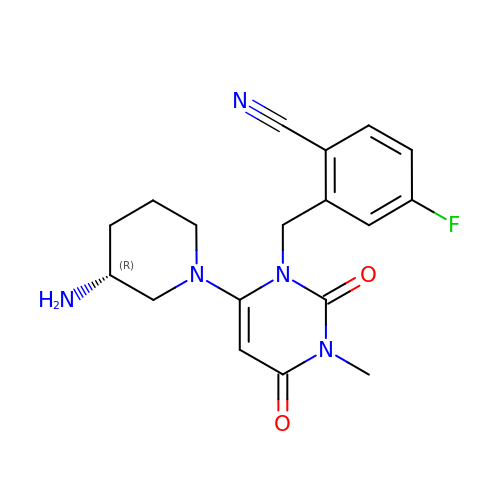2-[[6-[(3~{R})-3-azanylpiperidin-1-yl]-3-methyl-2,4-bis(oxidanylidene)pyrimidin-1-yl]methyl]-4-fluoranyl-benzenecarbonitrile | C18 H20 F N5 O2 | IWYJYHUNXVAVAA-OAHLLOKOSA-N1-BUTANE BORONIC ACID | C4 H11 B 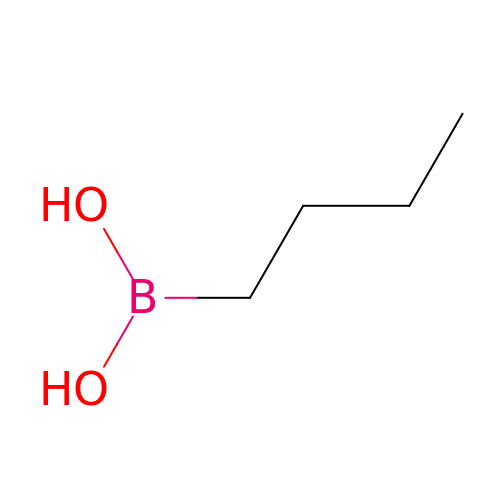O2 | QPKFVRWIISEVCW-UHFFFAOYSA-N> MNLAEKMYKAGQIEFAKGNYETAIIAYTLALLKDPNNAEAWYNLGEAYLALGNYEEAIEAYQKALELDPNNAEAWYNLGEAYL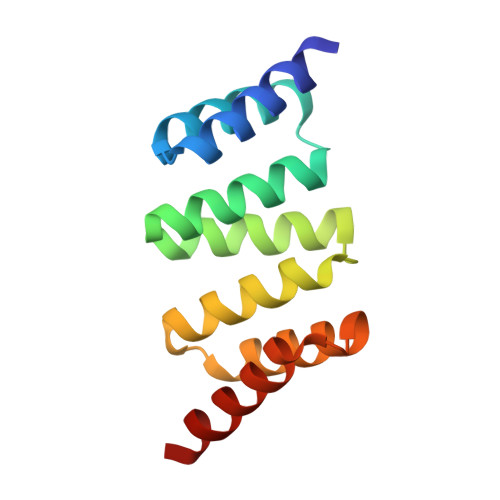ALGDYDNAIEAFTKALELDPNNKTAKAGLKLAKEKKALE> MGSDKIHHHHHHENLYFQGMILGIDVGGTSVKFGLVTPEGEIQNATRFMTADWVNGIGFVESMKLEIGNFLKQYPIVKGVGIGWPGLVSLDRTKVILLPNIPSVVNVPIVEILRSEFPHIHFKIENDAKCAALGEYYFGENKRMQTFILLALGTGVGSGVMMNG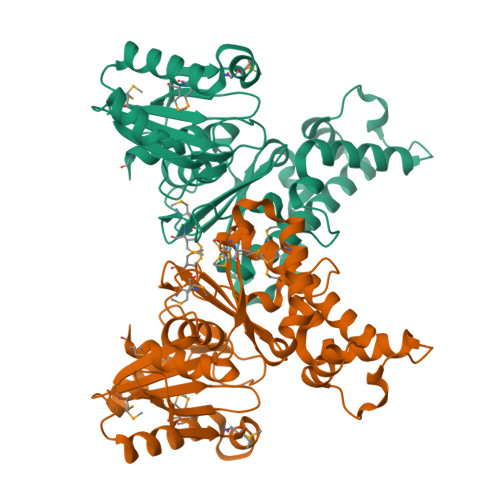KLFIGGRGNGTEVGHMLTTRGKSLENQVGINHLIAYTHEQLALDVAKKSSLHTIAELSPKVIADHAAQGDALALAVWADIGTIIGESLVNIVRVMDLNNILLGGGISGAFDYFVPNLKKAMLEHLPTYYTDDMYIGKATLENDAGLLGAAGLIMEAI>MVEPASIAELSRAEQLGKDQDAVRATVKEYYGETLKTSNDLRTSACTAAKAPPPAVRAALADVPTEVKEKFWGCGNPIPAGIEGLRVLDLGAGSGRDAYVAAKLVGEKGSVTGVDMTPAQLEVAISHADAYARDKLGYGKSNMTFIQGEIEYLDRAGLEDSSFDLVISNCVINLSPDKARVLSEAYRVLAPGGEMHFSDV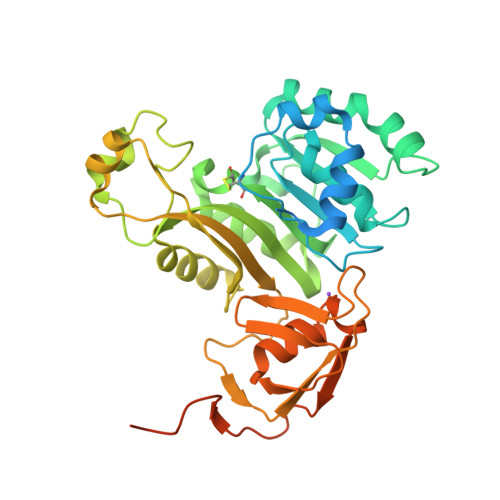YVDRRLPQSVRSHPVLLGECLAGALYNNDFIRLARKVGFTDPRQLEAEEIQIHDAELRDQVGEARFYSITYRLFKVPGQIEDLAEDYGQVAVYKGTIPGHSHAYDLDDHHRFVTNKPMLVAGNTASMVGESYLAPHFTIIGDRAVHYGQFDASGPKTTTGGAASPSNSAGAAGPGGAAALEHHHHHH[2x]In this work, we engineer EUGO, a VAO-type oxidase, to catalyze the selective dehydrogenation of 4-n-propylguaiacol to isoeugenol. Similar to VAO, EUGO is active on various 4-substituted phenols and contains a covalently bound FAD. The oxidation of 4-alkylphenols starts with a hydride transfer from the Cα atom of the substrate to the N5 of the flavin cofactor. Consequently, a p-quinone methide is formed and stabilized in the active site. This reactive intermediate can subsequently be hydroxylated by the base-catalyzed attack of water, or tautomerise to the dehydrogenation product.

To shed light on the effects of the introduced mutations on the enzyme structure, the crystal structure of the S394V-EUGO5X mutant in complex with 4-n-propylguiacol was solved at 2.9 Å resolution. The asymmetric unit comprises eight enzyme subunits forming four compact dimers. The overall three-dimensional structure of the mutant is virtually identical to that of the wild protein as revealed by an RMSD of 0.49 Å for 526 Cα atoms. The pattern emerging upon investigating these stabilizing mutations is clear: four of them (S81H, A423M, H434Y, S518P) create a better side chain packing by presenting bulkier or rigid aliphatic groups, whilst the fifth mutation (I445D) substitutes a hydrophobic residue with a charged one on the protein surface, and might contribute to overall stability by preventing protein aggregation and/or exposing a more hydrophilic side chain in direct contact with the solvent. The sixth (S394V) mutation of S394V-EUGO5X promotes enhanced chemoselectivity towards isoeugenol formation by favouring substrate dehydrogenation over hydroxylation. V394 is located at the entrance of the cavity where the substrate binds. Notably, this position represents the connection point between the active site and the wide chamber located at the subunit interface, which may comprise the entry passage of the water molecule which is used by EUGO to hydroxylate the reactive quinone methide intermediate. Therefore, a reasonable explanation for the higher chemoselectivity and reduced hydroxylation featured by the S394V-EUGO5X mutant is that the more hydrophobic and tightly sealed cavity of the S394V enzyme may hinder the accessibility of the Cα atom of the p-quinone methide intermediate to water, limiting the formation of the unwanted alcohol side-product. Specifically, careful inspection of the electron density revealed that the substrate is covalently bound to FAD in two of the eight crystallographic subunits present in the asymmetric unit, whilst in the other chains, the ligand was found to be non-covalently bound. By comparing the subunits with covalent and non-covalent bound substrates, we found that covalent binding is associated with a 20° tilting of the bound substrate.

>[8x]MTRTLPPGVSDERFDAALQRFRDVVGDKWVLSTADELEAFRDPYPVGAAEANLPSAVVSPESTEQVQDIVRIANEYGIPLHPVSTGKNNGYGGAAPRLSGSVIVKTGERMNRILEVNEKYGYALLEPGVTYFDLYEYLQSHDSGLMLDCPDLGWGSVVGNTLDRGVGYTPYGDHFMWQTGLEVVLPQGEVMRTGMGALPGSDAWQLFPYGFGPFPDGMFTQSNLGIVTKMGIALMQRPPASQSFLITFDKEEDLEQIVDIMLPLRINMAPLQNVPVLRNIFMDAAAVSKRTEWFDGDGPMPAEAIERMKKDLDLGFWNFYGTLYGPPPLIEMYYGMIKEAFGKIPGARFFTHEERDDRGGHVLQDRHKINNGIPSLDELQLLDWVPNGGHIGFVPVSAPDGREAMKQFEMVRNRANEYNKDYMAQFIIGLREMYHVCLFIYDTADPEAREEILQMTKVLVREAAEAGYGEYRTHNALMDDVMATFNWGDGALLKFHEKIKDALDPNGIIAPGKSGIWPQRFRGQNL> APAILLVDDEPHSLAAMKLALEDDFDVLTAQGAEAAIAILEEEW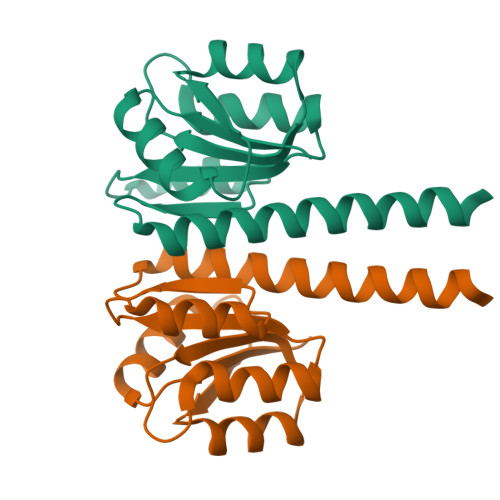VQVIICEQRMPGRTGVDFLTEVRERWPETVRIIITGYTDSASMMAAINDAGIHQFLTKPWHPEQLLSSARNAARMFTLARENERLSLEMRLLERP>[2x]FQGAMGSRVVILFTDIEESTALNERIGDRAWVKLISSHDKLVSDLVRRQSGHVVKSQGDGFMVAFARPEQAVRCGIELQRALR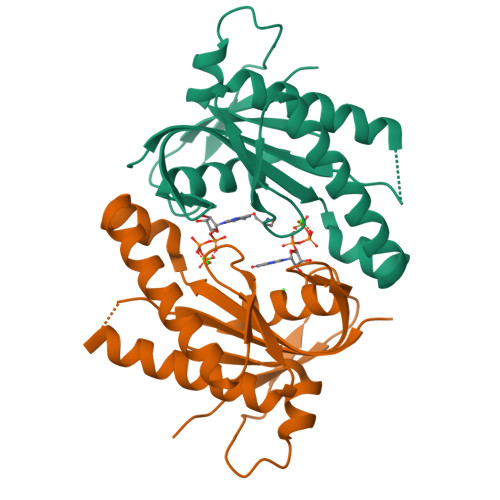RNANRKRHEEIRVRIGIHMGRSVRRGDDLFGRNVAMAARVAAQAAGGEILVSQPVRDALSRSDGIRFDDGREVELKGFSGTYRLFAVLASPDPG> GSHMAKEEIIWESLSVDVGSQGNPGIVEYKGVDTKTGEVLFEREPIPIGTNNMGEFLAIVHGLRYLKERNSRKPIYSDSQTAIKWVKDKKAKSTLVRNEETALIWKLVDEAEEWLNTHTYET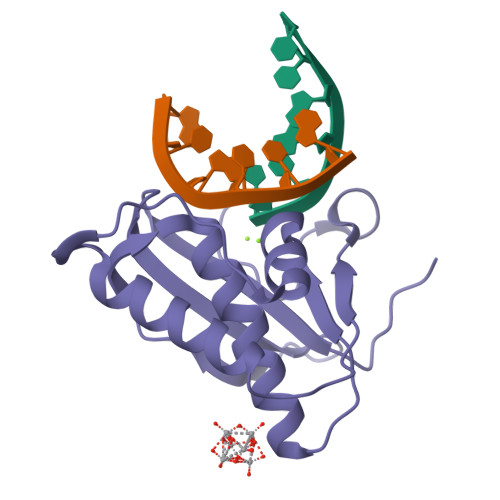PILKWQTDKWGEIKANYGRK> GAMGSGIPMEACPHIRYAFQNDKLLLQQASVGRLTLVNKTTILLRPMKTTTVDLGLYARPPEGHGLMLWGSTSRPVTSHVGIIDPGYTG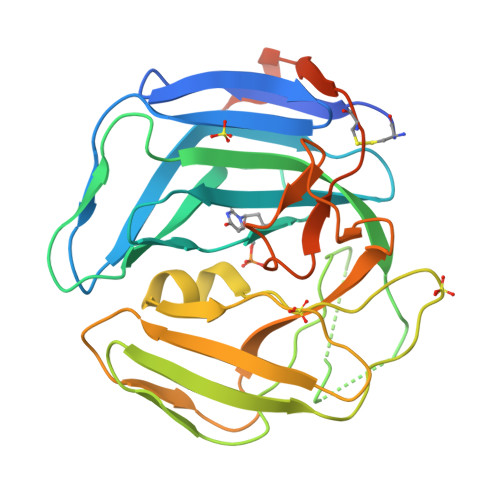ELRLILQNQRRYNSTLRPSELKIHLAAFRYATPQMEEDKGPINHPQYPGNVGLDVSLPKDLALFPHQTVSVTLTVPPPSIPHHRPTIFGRSGLAMQGILVKPCRWRRGGVDVSLTNFSDQTVFLNKYRRFCQLVYLHKHHLTSFYSPHSDAGVLGPRSLFRWASCTFEEVPSLAMGDSGLSEALEGRQGRGFGSSGQ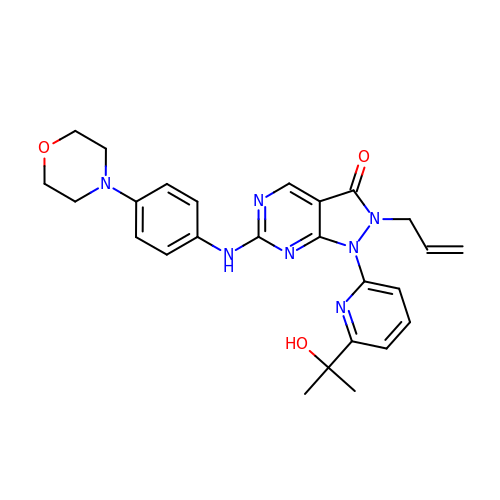1-[6-(2-hydroxypropan-2-yl)pyridin-2-yl]-6-{[4-(morpholin-4-yl)phenyl]amino}-2-(prop-2-en-1-yl)-1,2-dihydro-3H-pyrazolo[3,4-d]pyrimidin-3-one | C26 H29 N7 O3 | TVOBVNNUECNRHY-UHFFFAOYSA-N>GARPT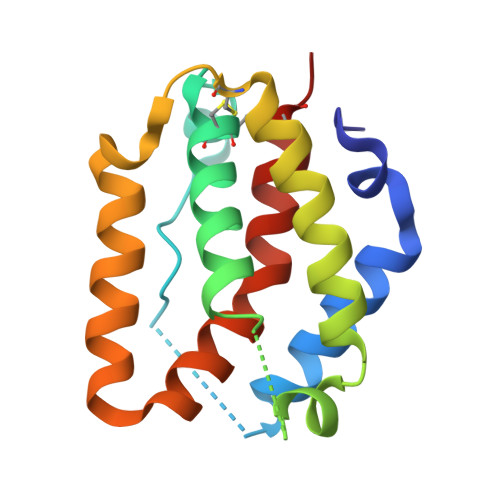PLDSSATWNDLAAMTDTARNEDDHETRLLPYFSHDMLQEEGSCCINARILKYYVNHVLESDEHTDMKYPMIRNVREGLHRVEQELQNHCKHDYSSHPLVKQFKRNYHASAIMDLAAARNKAIGETNTLYHYLFESCTPK[4x]>CACGUG[2x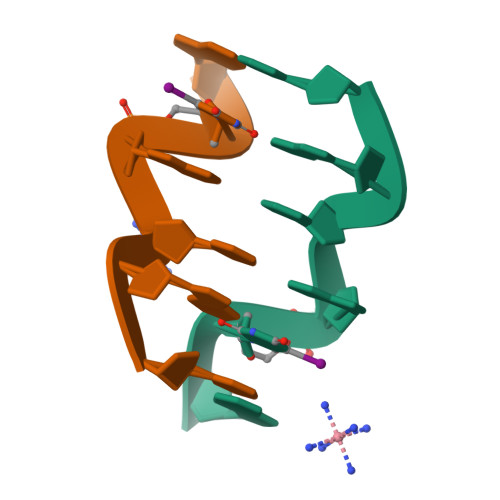]> MGSSHHHHHHSQDPNSISTTMSSYSIQQSQKMLTQLQIDYATNTSSNTVVAYLHNVGETTISYLQNSVV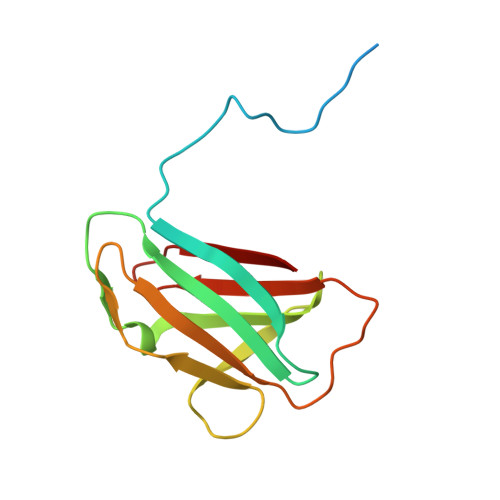YFGPNGQLQPVGYNSGSSPYWTVTSNSLQPGSKVKIIIYLSSPLSSNQYYTIQIVTPNGYTVSYMF>[2x]MGSSHHHHHHSSGRENLYFQGMATITLERDGLQLVGTREEPFGEIYDMAIIFHGFTANRNTSLLREIANSLRDENIASVRFDFNGHGDSDGKFENMTVLNEIEDANAILNYVKTDPHVRNIYLVGHAQGGVVASMLAGLYPDLIKKVVLLAPAATLKGDALEGNTQGV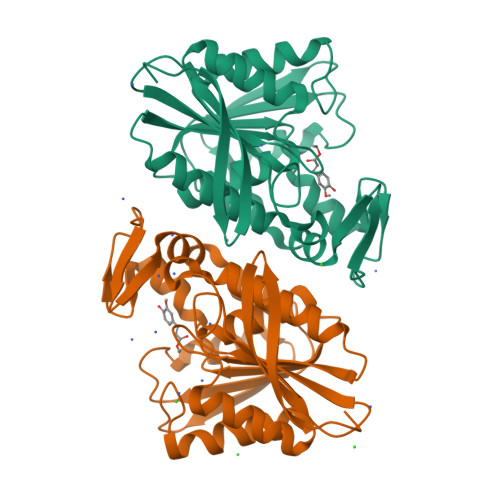TYNPDHIPDRLPFKDLTLGGFYLRIAQQLPIYEVSAQFTKPVCLIHGTDDTVVSPNASKKYDQIYQNSTLHLIEGADHCFSDSYQKNAVNLTTDFLQNNNAF>[5x]MDKSLFYNPQKMLSYDRILNFVIGARGIGKSYAMKVYPINRFIKYGEQFIYVRRYKPELAKVSNYFNDVAQEFPDHELVVKGRRFYIDGKLAGWAIPLSVWQSEKSNAYPNVSTIVFDEFIREKDNSNYIPNEVSAL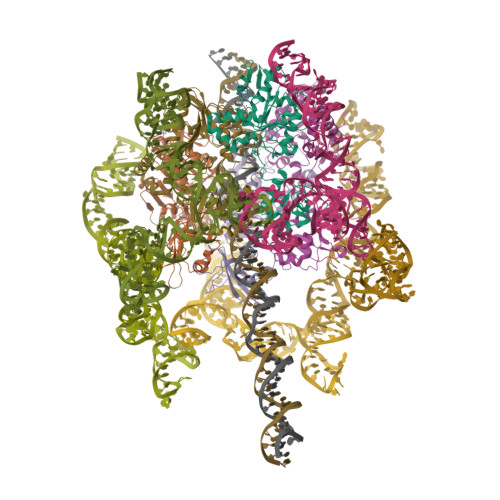LNLMDTVFRNRERVRCICLSNAVSVVNPYFLFFNLVPDVNKRFNVYDDALIEIPDSLDFSSERRKTRFGRLIDGTEYGEMSLDNQFIGDSQVFIEKRSKDSKFVFSIVYNGFTLGVWVDVNQGLMYIDTAHDPSTKNVYTLTTDDLNENMMLITNYKNNYHLRKLASAFMNGYLRFDNQVIRNIAYELFRKMRIQ The Ton complex is composed of three proteins ExbB, ExbD and TonB located in the inner membrane. It utilizes PMF to take up diverse compounds such as iron-loaded siderophores, haem, and vitamin B12 through outer membrane receptors. ExbB has three TM helices with a large cytoplasmic domain, and both ExbD and TonB are predicted to have single TM helices and a compact periplasmic domain. ExbB and ExbD together form a proton channel, and isolated ExbBD complexes show ion conductivity and cation selectivity in vitro.

Purified samples actually contain a significant amount of ExbD. To identify ExbD in the complex, we carried out 3D reconstruction from the cryo-EM images of the samples at pH 8.0 by single particle analysis (Supplementary file 1-Table S2). Starting from a reference map filtered to 30 Å resolution from the atomic model of the ExbB hexamer, a 3D structure was determined at 6.7 Å resolution with Bayesian-based algorisms implemented in RELION. Nonetheless, the map clearly resolves all α-helices and loops in the ExbB hexamer except for small parts of the loops at the periplasmic and at the cytoplasmic ends. The map also reveals three rod-like densities inside the channel, which likely correspond to the TM helices of three ExbD molecules. The helices fit snugly into the hexamer channel, with the arrangement off-centre and asymmetrical. Indeed, the rod-like densities disappear if 3-fold symmetry is enforced. We docked this domain of ExbD in the cryo-EM map, and the dimension of the mass in the periplasm is such that it accommodates three domain structures well. In contrast, each subunit in the fitted model (ExbB6ExbD3TM) is gradually dislocated by 1 ~ 3 Å from the membrane plane downwards towards the cytoplasmic side in the cryo-EM structure. The ExbB hexamer and ExbD trimer complex has a ~5.5 Å pore, which fits with the reported pore size of cation channels. Significantly, the cryo-EM structure shows that each of the subunits of the hexamer are slightly shifted downwards with respect to the prior adjacent molecule, resulting in a downward spiral of the hydrophobic ExbB wall that leads to the Asp 25 residues of the trimer.

>[6x]MGNNLMQTDLSVWGMYQHADIVVKCVMIGLILASVVTWAIFFSKSVEFFNQKRRLKREQQLLAEARSLNQANDIAADFGSKSLSLHLLNEAQNELELSEGSDDNEGIKERTSFRLERRVAAVGRQMGRGNGYLATIGAISPFVGLFGTVWGIMNSFIGIAQTQTTNLAVVAPGIAEALLATAIGLVAAIPAVVIYNVFARQIGGFKAMLGDVAAQVLLLQSRDLDLEASAAAHPVRVAQKLRAG;>NVTPFIDVMLVLLIIFMVAAPL[3x]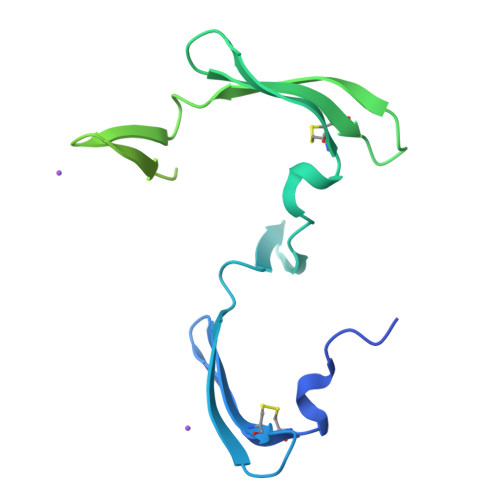> GHHHHHHIEGRLGKFSQTCYNSAIQGSVLTSTCERTNGGYNTSSIDLNSVIENVDGSLKWQPSNFIETCRNTQLAGSSELAAECKTRAQQFVSTKINLDDHIANIDGTLKYEGGSGGGGSGGLGKFSQTCYNSAIQGSVLTSTCERTNGGYNTSSIDLNSVIENVDGSLKWQPSNFIETCRNTQLAGSSELAAECKTRAQQFVSTKINLDDHIANIDGTLKYE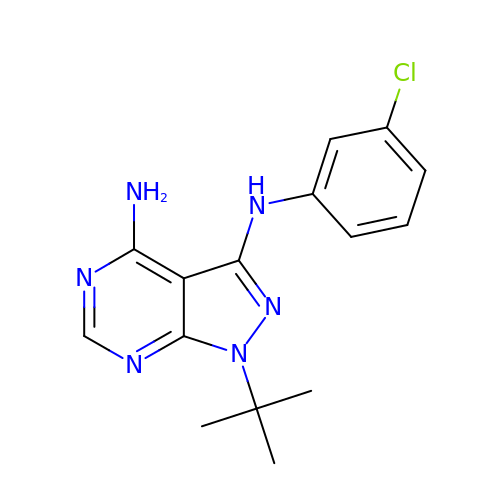1-tert-butyl-N~3~-(3-chlorophenyl)-1H-pyrazolo[3,4-d]pyrimidine-3,4-diamine | C15 H17 Cl N6 | GOBSWYSUEYZTQX-UHFFFAOYSA-N>MAEKPKLHYFNARGRMESTRWLLAAAGVEFEEKFIKSAEDLDKLRNDGYLMFQQVPMVEIDGMKLVQTRAILNYIASKYNLYGKDIKERALIDMYIEGIADLGEMILLLPVCPPEEKDAKLALIKEKIKNRYFPAFEKVLKSHGQDYLVGNKLSRADIHLVELLYYVEELDSSLISSFPLLKALKTRISNLP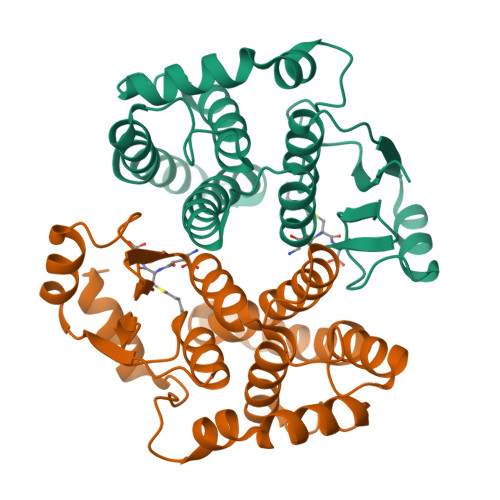TVKKFLQPGSPRKPPMDEKSLEEARKAFRF[2x]> GDSLSIHQLAAQGELDQLKEHLRKGDNLVNKPDERGFTPLIWASAFGEIETVRFLLEWGADPHILAKERESALSLASTGGYTDIVGLLLERDVDINIYDWNGGTPLLYAVRGNHVKCVEA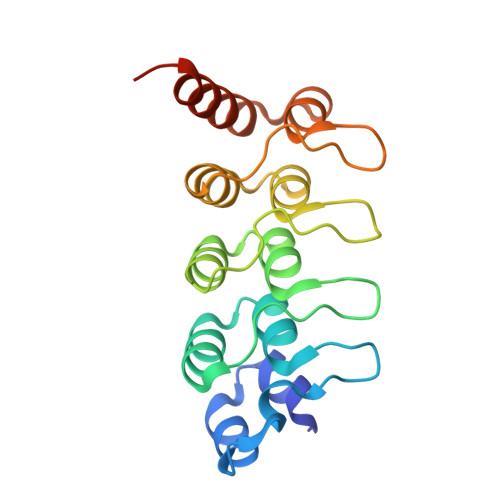LLARGADLTTEADSGYTPMDLAVALGYRKVQQVIENHILKLFQSNLVPADPE>MSRQASRLDAKKVNSEFLTLTYGALVTQMLRDFENAEDVNKQLERIGYNMGMRLIEDFLARTSAPRCLEMRETADRIQQAFRIYLNIQPTISNWSPASDEFSLVFDSNPLTEFVELPPDLTNLRYSAILSGCIRGALEMVQLEVQCWFVQDQLKGDNVTELRVKFVRRLEEVIPAGED[2x];> MSEEILFDCLHAEIVNYCLDSNKEHDLATLEYIGFTTGYRLIERLTREVSRFKDELETMKFICTDFWMLIYKKQVDNLRTNNHGMYVVQDKA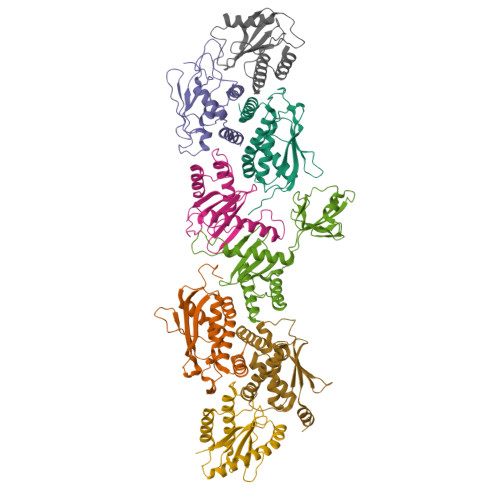FRFLTRISPGTKQLEHAPKFVAFTCGLVRGALSNLGINSTVTAEVQSIPACKFHIEVNRN;> MTIFNLYIFDKFGTLLHYAEWNRTKKSGITREEEAKLTYGMLFSIKSFVSKISPHDPKEGFLYYKTNRYALHYLETPSGLKFVLNTDTTAINVKELLQQLYAKVWVEFVVRDPLWTPGTVVTSELFQSKLDEFVRQSPIFGIRNI;> MIIYGVYIVSKSGGLIFNLDNNVPRIEHEKTFTYPLDLVLDYDSKKVSVSFNRKDGINVGHVLVAVNGMPVNGVTLDDGRDVRTTLDAPENYPINLKFSRPKMTTNEKIFLASMFYPLFAIASQLSPEPKSSGIEILEADTFTLHCFQTLTGIKFIIISETGLNGIDLLLRKVYELYSDYVLKNPFYSLEMPIRCELFDNKLQELLAQVEKTGISNIDK;> MSTYYFVIVGQNDNPIYEKEFSTVNKELRKEDHRHLTQFIAHAALDLVDEHKWKTANMQLKSIDRFNQWFVSAFITASQIRFIIVHDNKNDEGIKNFFNEMYDTYIKNSMNAFYRINTPIKSPMFEKKSEIFGRKYLLS;> MEKLEALKISSMRPRSNILDRPLSKGKTEVSQSIVALLFSEIVQYSQSRVFTVPELQTRLHDLGQDVGTRIIDLYFVRERSSKRETKLTQMLLFVKTTVWKNLFGKEAEKLEHANDDERTYYIIEKEPLVNTFISVPKDKGSLNCANFTAGIVEAVLTNCGFPCKVTAHWHKGTTYMVKFEDFVIARDKQMEEK;> MAFCIAVIGKDNAPLYLTTSDMEQELELQYHVNAALDVVEEKCLIGKGAPESKELYLGLLYSTENHKIYGFVTNTRVKFIVVIDSSNVALRENEVRAIFRNLHLLYTDAICNPFYIPGESLTSKKFDRAVQKLMSGTA Enolase, a ubiquitous enzyme, catalyzes the reversible conversion of 2-phospho­glycerate (2PG) to phospho­enolpyruvate (PEP) in the glycolytic pathway of organisms of all three domains of life. Here we present structural snapshots of Mycobacterium tuberculosis (Mtb) enolase in apo, PEP-bound and two 2PG-bound forms as it catalyzes the conversion of PEP to 2PG. MtEno has a topology similar to other enolase structures, a smaller N-terminal domain and a larger C-terminal domain. The crystal and the cryoEM structures (enzyme in solution, frozen) along with the biochemical studies clearly demonstrate that the functional unit of MtEno is an octamer.

Tautomerization resonance is accelerated on acidification of the carboxyl group of 2PG which is accomplished through its lone-pair-mediated coordination with both the Mg2+ ions and the transfer of a proton from His154 onto the nearest oxygen linked to the phosphate moiety. To find out if the exact reverse of this reaction occurs during the conversion of PEP to 2PG, we systematically mutated each of the residues Ser42, Asp241, Glu163, Glu204 and Lys335 to alanine, compared their activity with wild type MtEno, and elucidated the structures of three of them [Figs. 4(a) and 4(b)].

> MHHHHHHMPIIEQVRAREILDSRGNPTVEVEVALIDGTFARAAVPSGASTGEHEAVELRDGGDRYGGKGVQKAVQAVLDEIGPAVIGLNADDQRLVDQALVDLDGTPDKSRLGGNAILGVSLAVAKAAADSAELPLFRYVGGPNAHILPVPMMNILNGGAHADTAVDIQAFMVAPIGAPSFVEALRWGAEVYHALKSVLKKEGLSTGLGDEGGFAPDVAGTTAALDLISRAIESAGLRPGADVALALDAAATEFFTDGTGYVFEGTTRTADQMTEFYAGLLGAYPLVSIEDPLSEDDWDGWAALTASIGDRVQIVGDDIFVTNPERLEEGIERGVANALLVKVNQIGTLTETLDAVTLAHHGGYRTMISHRSGETEDTMIADLAVAIGSGQIKTGAPARSERVAKYNQLLRIEEALGDAARYAGDLAFPRFACETK(3~{R})-8-methoxy-3-methyl-3,6-bis(oxidanyl)-2,4-dihydrobenzo[a]anthracene-1,7,12-trione 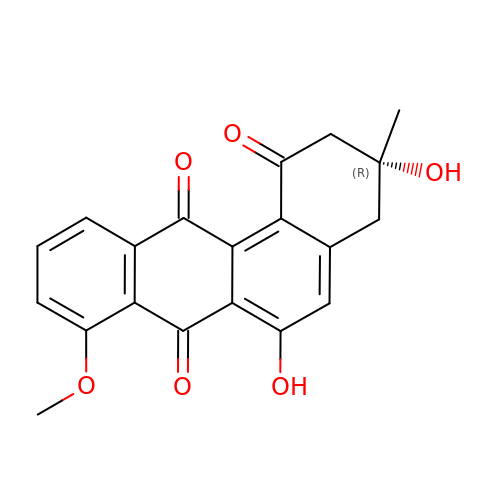| C20 H16 O6 | LQIPGPPZCXJWKY-HXUWFJFHSA-N> KQLASKAA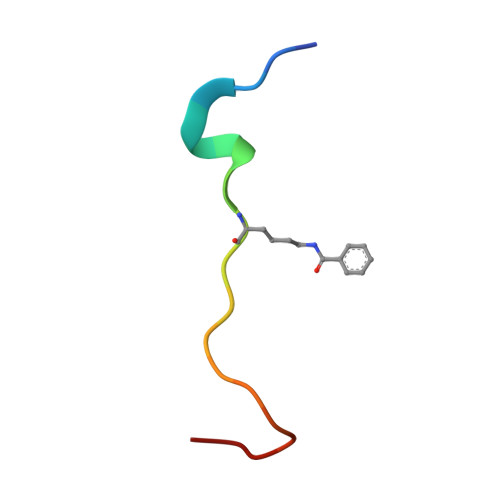RKSAPSTGGVKY> P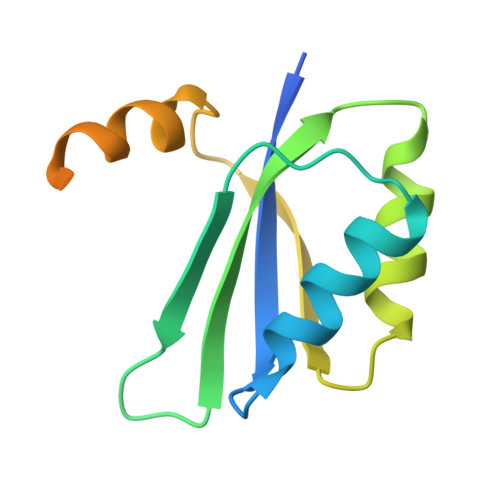MQNTTHDNVILELTVRNHPGVMTHVCGLFARRAFNVEGILCLPIQDSDKSHIWLLVNDDQRLEQMISQIDKLEDVVKVQRNQSDPTMFNKIAVFFQASTAATSAAATSAAATSAAATSAAATSAAS N-{[(2E)-2-(pyridin-4-ylmethylidene)hydrazino]carbonothioyl}-beta-D-glucopyranosylamine | C13 H18 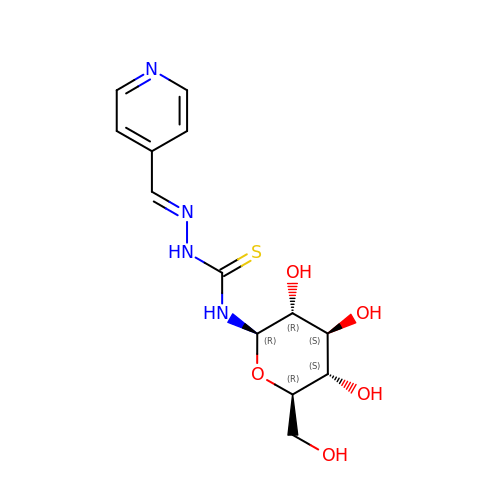N4 O5 S | KHZWKRXKMLEULJ-XYUJZHSNSA-N>[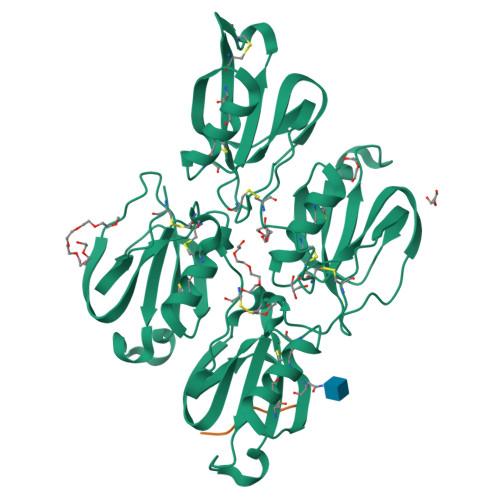2x]RSHHHHHHGCLTQLYENAFFRGGDVASMYTPNAQYCQMRCTFHPRCLLFSFLPASSINDMEKRFGCFLKDSVTGTLPKVHRTGAVSGHSLKQCGHQISACHRDIYKGVDMRGVNFNVSKVSSVEECQKRCTNNIRCQFFSYATQTFHKAEYRNNCLLKYSPGGTPTAIKVLSNVESGFSLKPCALSEIGCHMNIFQHLAFSDVDVARVLTPDAFVCRTICTYHPNCLFFTFYTNVWKIESQRNVCLLKTSESGTPSSSTPQENTISGYSLLTCKRTLPEPCHSKIYPGVDFGGEELNVTFVKGVNVCQETCTKMIRCQFFTYSLLPEDCKAEACKCFLRLSMDGSPTRIAYGTQGSSGYSLRLCNTG;>TQSDDDWIPDIQIDPNGLSFNPISDFPDT[2x]>[4x]SALADDLKKWVGETFTGKWEVQETTSVPNPEDLRLNSNHAKDLKAATVLYADLDGSTDMVNTKKWQFSAQIYKTFLKCASDIIRDEGGNITAY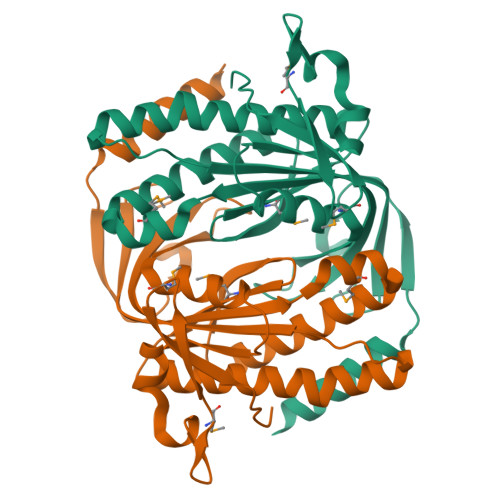DGDRVMAVFTGNSKNTSAARCALKINSAVLDIIQPAIAKKWQTDFVLRHVVGIDTSQLRTARIGIRGDNDLVWIGRAANYAAKLTNLAGKPTRITADVYNKLADKLKYANGVDMWAPEHWDDMGIWTYTSTWKWTV> SQETFEEKYRLSPT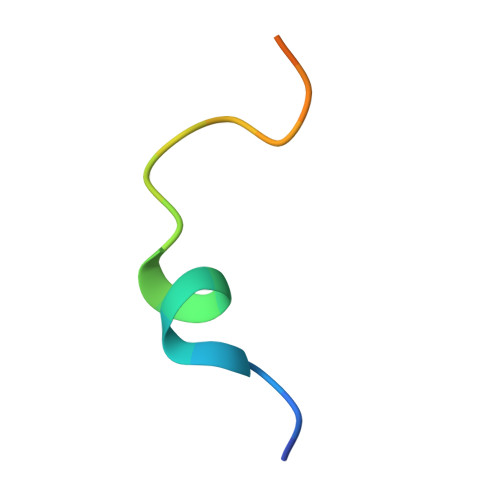LSSTKGH>GAAEQTGLKASQDNVNIPDSTFKAYLNGLLGQSSTANITEAQMNSLTYITLANINVTDLTGIEYAHNIKDLTINNIHATNYNPISGLSNLERLRIMGKDVTSDKIPNLSGLTSLTLLDISHSAHDDSILTKINTLPKVNSIDLSYNGAITDIMPLKTLPELKSLNIQFDGVHDYRGIEDFPKLNQLYAFSQTI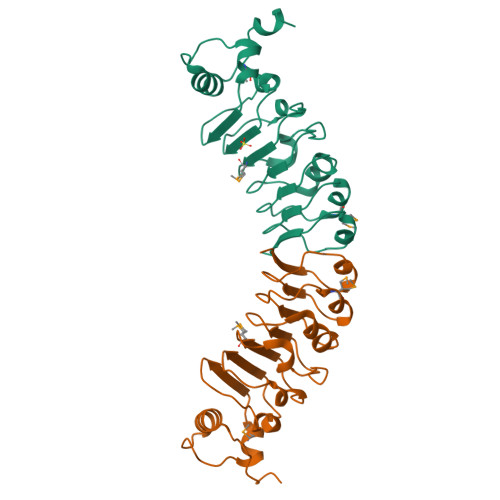GGKK[2x]> AKMAFTLADRVTEEMLADKAALVVEVV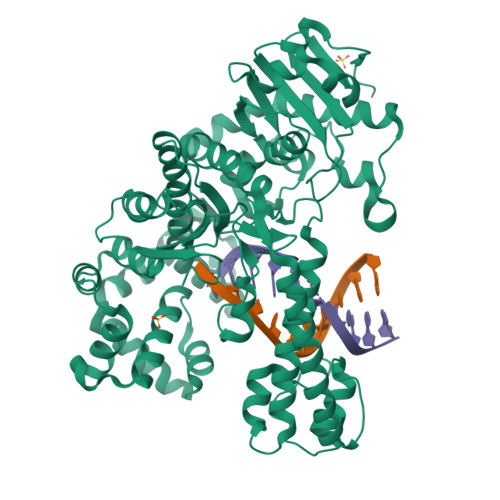EENYHDAPIVGIAVVNEHGRFFLRPESALADPQFVAWLGDETKKKSMFDSKRAAVALKWKGIELCGVSFDLLLAAYLLDPAQGVDDVAAAAKMKQYEAVRPDEAVYGKGAKRAVPDEPVLAEHLVRKAAAIWALERPFLDELRRNEQDRLLVELEQPLSSILAEMEFAGVKVDTKRLEQMGKELAEQLRTVEQRIYELAGQEFNINSPKQLGVILFEKLQLPVLKKTKTGYSTSADVLEKLAPYHEIVENILHYRQLGKLQSTYIEGLLKVVRPDTKKVHTIFNQALTQTGRLSSTEPNLQNIPIRLEEGRKIRQAFVPSESDWLIFAADYSQIELRVLAHIAEDDNLMEAFRRDLDIHTKTAMDIFQVSEDEVTPNMRRQAKAVNKGIVYGISDYGLAQNLNISRKEAAEFIERYFESFPGVKRYMENIVQEAKQKGYVTTLLHRRRYLPDITSRNFNVRSFAERMAMNTPIQGSAADIIKKAMIDLNARLKEERLQARLLLQVHDELILEAPKEEMERLCRLVPEVMEQAVTLRVPLKVDYHYGSTWYDAK> MADIIADADSPAKITIKANKLKDLKDYVDDLKTYNNTYSNVVLEHHHH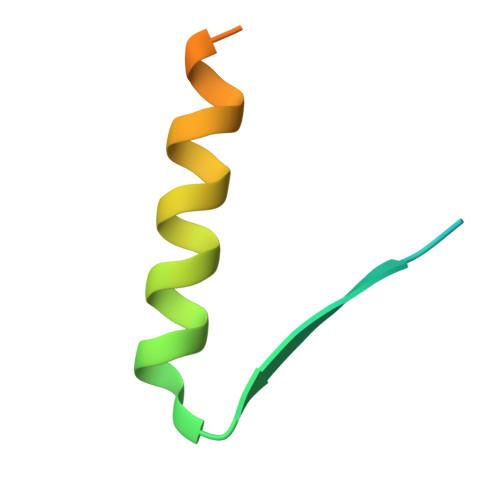HH> GSKKIFKPEELRQALMPTLEALYRQDPESLPFRQPVDPQLLGIPDYFDIVKNPMDLSTIKRKLDTGQYQEPWQYVDDVWLMFNNAWLYNRKTSRVYKFCSKLAEVFEQEIDPV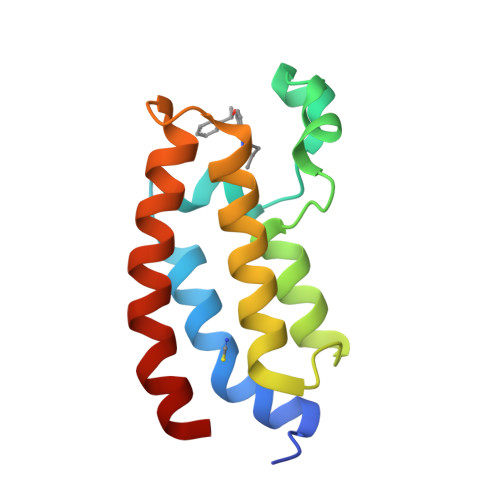MQSLG> MRGSHHHHHHTDQFTMEQNPQSQLKLLVTRGKEQGYLTYAEVNDHLPEDIVDSDQIEDIIQMINDMGIQVMEEAPDADDLMLAENTADEDAAEAAAQVLSSVESEIGRTTDPVRMYMREMGTVELLTREGEIDIAKRIEDGINQVQCSVAEYPEAITYLLEQYDRVEAEEARLSDLITGFVDPNAEEDLAPTATHVGSELSQEDLDDDEDEDEEDGDDDSADDDNSIDPELAREKFAELRAQYVVTRDTIKAKGRSHATAQEEILKLSEVFKQFRLVPKQFDYLVNSMRVMMDRVRTQERLIMKLCVEQCKMPKKNFITLFTGNETSDTWFNAAIAMNKPWSEKLHDVSEEVHRALQKLQQIEEETGLTIEQVKDINRRMSIGEAKARRAKKEMVEANLRLVISIAKKYTNRGLQFLDLIQEGNIGLMKAVDKFEYRRGYKFSTYATWWIRQAITRSIADQARTIRIPVHMIETINKLNRISRQMLQEMGREPTPEELAERMLMPEDKIRKVLKIAKEPISMETPIGDDEDSHLGDFIEDTTLELPLDSATTESLRAATHDVLAGLTAREAKVLRMRFGIDMNTDYTLEEVGKQFDVTRERIRQIEAKALRKLRHPSRSEVLRS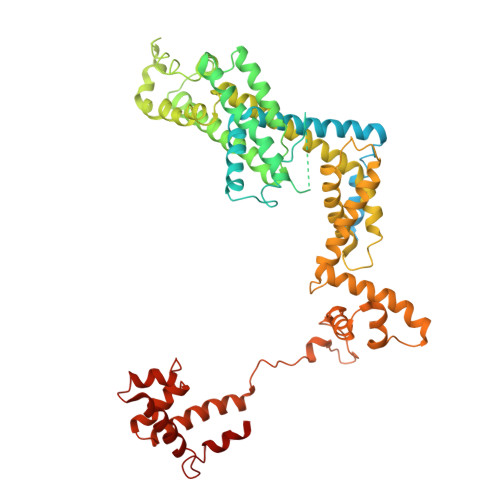FLDD>SYTLPSLPYAYDALEPHFDKQTMEIHHTKHHQTYVNNANAALESLPEFANLPVEELITKLDQLPADKKTVLRNNAGGHANHSLFWKGLKKGTTLQGDLKAAIERDFGSVDNFKAEFEKAAASRFGSGWAWLVLKGDKLAVVSTANLDSPLMGE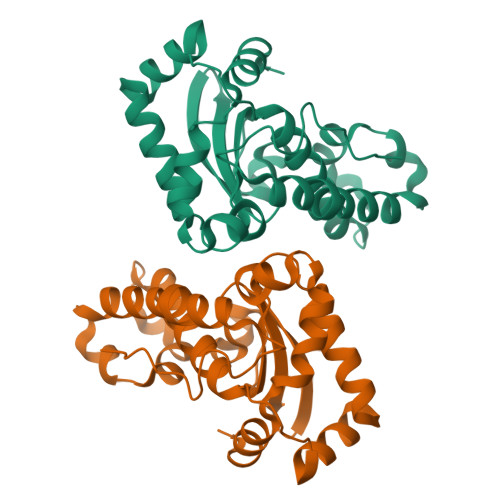AISGASGFPIMGLDVWEHAYYLKFQNRRPDYIKEFWNVVNWDEAAARFAAKK[4x]> PDSLFAGLVGEYYGTNSQLNNISDFRALVDSKEADATFEAANISYGRGSSDVAKGTHLQEFLGSDASTLSTDPGDNTDGGIYLQGYVYLEAGTYNFKVTADDGYEITINGNPVATVDNNQSVYTVTHASFTISESGYQAIDMIWWDQGGDYVFQPTLSADGG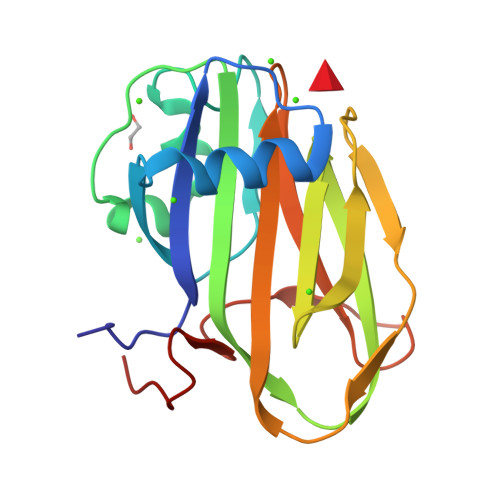STYFVLDSAILSSTGETPYT The rotating flagellar filament primarily functions as a propeller, acting as an Archimedean screw, and supercoiling of the filament is essential as rotations of a straight filament do not generate thrust. Here, we show the atomic cryo-electron microscopy structures for flagellar filaments from enterohemorrhagic Escherichia coli O157:H7, enteropathogenic E. coli O127:H6, Achromobacter, and Sinorhizobium meliloti, where the outer domains dimerize or tetramerize to form either a sheath or a screw-like surface. A shared feature in all four structures is the formation of symmetrical homodimers between the outer domains of flagellin subunits, with one outer domain rotated 180° relative to the other. These symmetrical dimers are the result of outer domains being able to adopt either an “up” or “down” conformation.

Similar to the S. meliloti flagellar filament, the EHEC O157:H7 flagellar filament has a dimer symmetry with two flagellins in the ASU, one with an up and one with a down outer domain conformation. The much larger EHEC H7 outer domains (D2, D3, and D4) interact with outer domains from three other subunits forming a mesh-like ODS. In addition to forming dimers with outer domains that are five and 11 subunits away, every EHEC H7 outer domain also pairs with an outer domain that is 27 subunits away. This long-range Sn:Sn + 27 dimer results in an observable 8-start helix on the surface of the sheathed filament in addition to a 3-start. The S. meliloti, EHEC O157:H7, and Achromobacter flagellar filament structures were solved using helical reconstruction to 3.7, 3.6, and 3.7 Å resolution, respectively. To investigate ODS function, we aimed to disrupt its formation by mutation of several key residues in the EHEC H7 Sn:Sn + 27 domain D4 dimer interface. Residues N319 and N323 in the EHEC H7 flagellin were chosen for mutagenesis. Two double mutants were constructed: N319F N323F (FF) and N319R N323R (RR) and mutant flagellar filaments isolated. Cryo-electron micrographs revealed that the FF mutant filament had a disrupted surface compared to that of wild-type EHEC H7. Soft agar (0.3%) motility assays revealed drastically reduced motility of cells with the FF and RR mutant flagellar filaments as compared to the wild-type H7.

>MAQVINTNSLSLITQNNINKNQSALSSSIERLSSGLRINSAKDDAAGQAIANRFTSNIKGLTQAARNANDGISVAQTTEGALSEINNNLQRIRELTVQATTGTNSDSDLDSIQDEIKSRLDEIDRVSGQTQFNGVNVLAKDGSMKIQVGANDGETITIDLKKIDSDTLGLNGFNVNGKGTITNKAATVSDLTSAGAKLNTTTGLYDLKTENTLLTTDAAFDKLGNGDKVTVGGVDYTYNAKSGDFTTTKSTAGTGVDAAAQAADSASKRDALAATLHADVGKSVNGSYTTKDGTVSFETDSAGNITIGGSQAYVDDAGNLTTNNAGSAAKADMKALLKAASEGSDGASLTFNGTEYTIAKATPATTTPVAPLIPGGITYQATVSKDVVLSETKAAAATSSITFNSGVLSKTIGFTAGESSDAAKSYVDDKGGITNVADYTVSYSVNKDNGSVTVAGYASATDTNKDYAPAIGTAVNVNSAGKITTETTSAGSATTNPLAALDDAISSIDKFRSSLGAIQNRLDSAVTNLNNTTTNLSEAQSRIQDADYATEVSNMSKAQIIQQAGNSVLAKANQVPQQVLSLLQG[44x]>GSHMADLSNSQNISPGAEPLILNLSSNIYSSDITQQIEV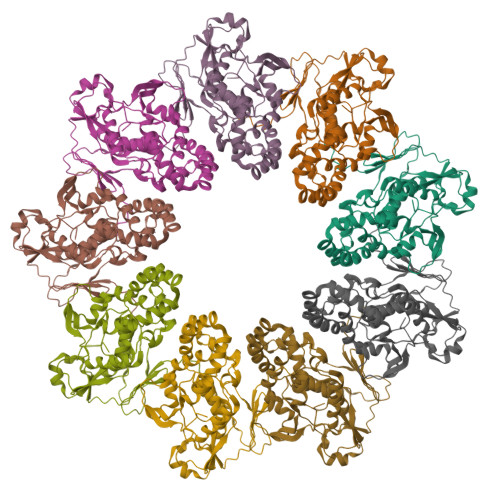MRWNFFEESGIPLPKIIVNPVKNNDSAIEFLLYQESIYKDTLIDDTVYFEAGHAEISFEFVQEKLSTNSIVYKTNKTNQQLAHLTGMDVYATTNDKITFLLKKLVLSNAKEFIGVQETRYLMDIMERKYNELVKELQRQLGLSKIVDILQRLVEENVSIRDLRTIFETLIFWSTKEKDVVILCEYVRIALRRHILGRYSVSGTLLNVWLIGSDIENELRESIRQTSSGSYLNISPERTEQIIGFLKNIMNPTGNGVILTALDIRRYVKKMIEGSFPSVPVLSFQEVGNNIELKVLGTVNDFRA[9x]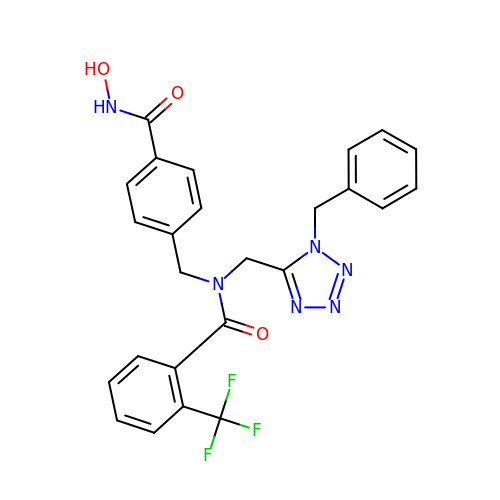N-[(1-benzyl-1H-tetrazol-5-yl)methyl]-N-{[4-(hydroxycarbamoyl)phenyl]methyl}-2-(trifluoromethyl)benzamide | C25 H21 F3 N6 O3 | MEWDNULKAXEKII-UHFFFAOYSA-N>[2x]RPMDNEAVQFGMSMGIGWNLGNQMDAHYDGCSYETGWGNKAATQQTFNGLAKAGFRSVRIPVTWMGHIGNAPTYAIERGWLDRVDELVHMAHKAGLIVIINIHHDGFGAADTPSKGSHWLDLPAAVASEERNQLIKQELTMIWLQIGKRFANDGEWLVFETLNEIQDGDWGNGNNRRDGGAQYRVLNEWNQVCVDAIRAAGGKNETRYIGVPGYVCNPDLTVENLVLPEDVVPNRLMVAVHSYDPWDYAGSAKYNEWGHTGKDVVPGVGEEAYVGMLNRLFNMYIRRGVPVYFGEFGAVRRASKADEEFRLYYFRYICKAMRDRRISALYWDNGNSKAGNDGFGVIDHATGRFIGNGEQAVRAMIDSWENNDPNYTLQSIYDSAPESSR

AC2aCel5A is an endo-acting cellulase that is encoded within the first reported cellulolytic PUL, originating from an uncultured Bacteroidetes phylotype. As previously reported, AC2aCel5A is an endoglucanase active on β-(1,4) glycosidic bonds between glucose units in soluble and insoluble cellulosic substrates and in linear β-glucans. The enzyme displays the typical (β/α)8 barrel structure associated with the GH5 family. The six closest structural homologues, which include all the biochemically characterized members of subfamily GH5_4, were identified using the Dali server17 and were used to produce a structure-based multiple sequence alignment using the PROMALS3D server. This allowed identification of the conserved catalytic residues, i.e. Glu172 and Glu303, acting as the catalytic acid and nucleophile/base, respectively.

The structure of AC2aCel5A was solved to 1.8 Å, and contained two molecules in the asymmetric unit. The final model comprised residues 9–397; no electron density was observed for the nine N-terminal residues nor for the final eight C-terminal residues, including the His6-tag. The native structure was solved to 1.8 Å resolution and revealed a narrow substrate-cleft, likely determining the specificity of the enzyme for linear and less substituted substrates. A surface projection shows the narrow groove stretching across the enzyme, with the active-site located in its center. A comparison of the active-site clefts of the GH5s shows that AC2aCel5A has a narrower active site cleft than its homologues, especially in the vicinity of the −3 to −1 sub-sites. This is primarily caused by the loop region between β3 and α3’ (red surface), which protrudes into the substrate-binding cleft and which is extended in AC2aCel5A, compared to the examined homologues (residues 115–126). Nonetheless, AC2aCel5A is unique in that it has an exceptionally narrow active site cleft, due to an extended loop region that seems well adapted to (only) acting on less-substituted β-glucans. AC2aCel5A contains a tryptophan “clamp” in its putative +1 and +2 subsites, analogous to what has been observed in other glycoside hydrolases acting on insoluble polysaccharides. Furthermore, in both the apo- and the complex structure, extra electron density was also observed close to, and between Trp178 and Trp254 in the substrate-binding cleft of both chain A and B.>[2x]MFKTTLCALLITASCSTFAAPQQINDIVHRTITPLIEQQKIPGMAVAVIYQGKPYYFTWGYADIAKKQPVTQQTLFELGSVSKTFTGVLGGDAIARGEIKLSDPTTKYWPELTAKQWNGITLLHLATYTAGGLPLQVPDEVKSSSDLLRFYQNWQPAWAPGTQRLYANSSIGLFGALAVKPSGLSFEQAMQTRVFQPLKLNHTWINVPPAEEKNYAWGYREGKAVHVSPG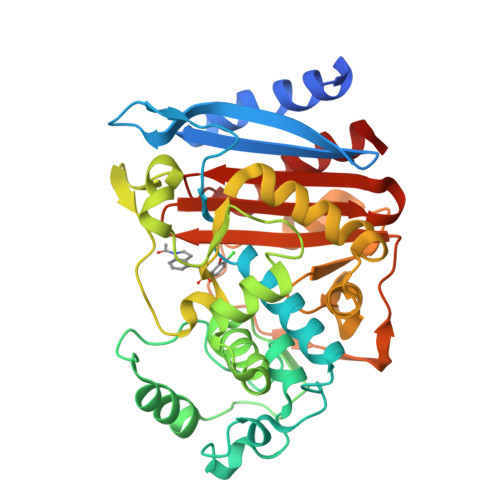ALDAEAYGVKSTIEDMARWVQSNLKPLDINEKTLQQGIQLAQSRYWQTGDMYQGLGWEMLDWPVNPDSIINGSDNKIALAARPVKAITPPTPAVRASWVHKTGATGGFGSYVAFIPEKELGIVMLANKNYPNPARVDAAWQILNALQ>SGKAPGSEGGSAPDGALTLGFAQVGAESGWRTANTESIKSAAEEAGVNLKFADANGEQEKQISAIRSFIQQGVDVIAFSPVVRTGWDAVLQETKNAGIPVILTDRAVDTQDTDVYKTFIGADFIEEGRRAGQWVADQYASATGPVNIVQLEGTTGADPAIDRKTGFAEGISKNPNLKIVASQTGDFTRSGGKQVMEAFLKSTPQIDVVFAQNDDMGLGAMEAIEAAGKKPGTDIKIVAVDATHDGMQALADGKFNYIVECNPLLGPELM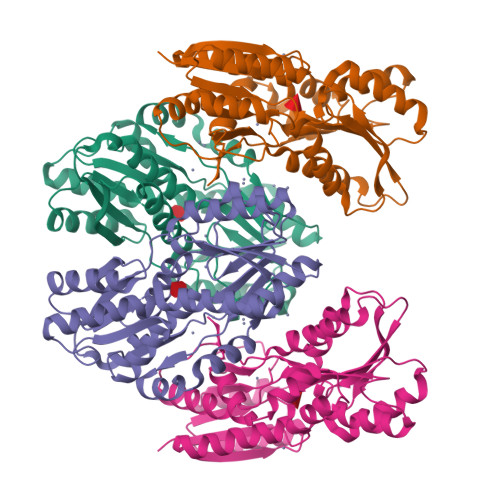DLAKKVAAGEPVPERVVTPDEAFDQAQAKAALPNRQYKLAAALEHHHHHH[2x]Here, we have used metagenome-based technologies to identify and characterize novel bacterial lipolytic enzymes which catalyze both hydrolysis and esterification reactions at temperatures above 70°C. Metagenomic libraries from enriched soil and water samples were constructed and screening revealed two novel lipases designated LipS and LipT which showed a high temperature optimum and also a high stability against thermal denaturation. LipS assumes the fold of a classical α/β hydrolase. The active site of LipS is formed by the catalytic triad S126, D227 and H257 with the catalytic serine located at the sharp γ-turn between β4 and αD. The position of the catalytic triad and the oxyanion hole (F58 and M127) at conserved topological sites clearly designates this newly characterized enzyme as a hydrolase.

The initial construct LipS-H6 in SG P42212 diffracted X-ray radiation to 2.80 Å resolution, while a second construct, LipS-WT, diffracted X-ray radiation to 1.99 Å resolution. Both constructs contain the native N-termini which are disordered until about residue 35. LipS displayed a dimeric character during purification by size exclusion chromatography. Consistent with this observation, the asymmetric units of LipS in SG P4 and P42212 contain one and two identical dimers, respectively. The structure of LipS was solved for two different constructs which crystallized in two different space groups. In the higher resolution SG P4, there is clear additional electron density immediately adjacent to the catalytic S126 and H257. In LipS in SG P42212, however, there is no such electron density. This excludes the possibility that the observed density results from expression in E. coli. We interpreted this residual density with spermidine, which was added during crystallization of LipS in SG P4 but not in SG P42212. Furthermore, data that the inserted domain assumes the same conformation with and without bound spermidine in structures of LipS suggests that this is rather a rigid structure. Identical conformations of the lid-domain, which covers the active site, in the absence and presence of a ligand, indicate that this domain may not undergo conformational rearrangements during the catalytic cycle.

>[2x]MSRKSRNCRNPPRSGDAQQRPRERSGSGMSTTPLQVLPGAEPLYSVGSRIGVLVSHGFTGSPQSMRFLAEGFARAGYTVATPRLTGHGTTPAEMAASTASDWTADIVAAMRWLEERCDVLFMTGLSMGGALTVWAAGQFPERFAGIMPINAALRMESPDLAALAFNPDAPAELPGIGSDIKAEGVKELAYPVTPVPAIKHLITIGAVAEMLLPRVKCPALIIQSREDHVVPPHNGELIYNGIGSTEKELLWLENSYHVATLDNDKELILERSLAFIRKHSKLAAALEHHHHHH>M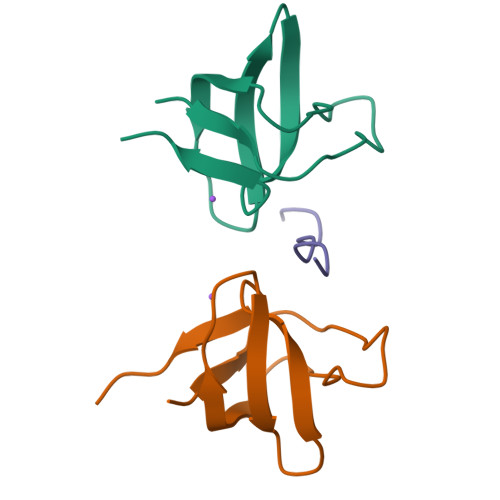VEAIVEFDYQAQHDDELTISVGEIITNIRKEDGGWWEGQINGRRGLFPDNFVREIKK[2x];> PARPPKPRPRR Itaconate, which is an unsaturated dicarboxylic acid produced by the decarboxylation of cis-aconitate, is an intermediate metabolite in the tricarboxylic acid cycle and is a striking example of a small metabolite that regulates enzyme activity for cell growth and survival. Initial studies of itaconate production in fungi indicate that the decarboxylation of cis-aconitate to generate itaconate was catalyzed by a ~ 55 kDa protein, which was called cis-aconitate decarboxylase (CAD). In mammals, high amounts of itaconate are produced by macrophages activated by lipopolysaccharide, which is a major pathogen-associated molecular pattern in gram-negative bacteria. Our structural investigation of IRG1 from B. subtilis (bsIRG1) shows that bsIRG1 exhibits the typical fold of the MmgE/PrpD family containing two distinct domains, a helical domain and a lid domain.

The 1.78 Å crystal structure of full-length bsIRG1 was elucidated by using the molecular replacement (MR) method. There were two molecules in the asymmetric unit, chains A and B, both constructed from residues 3 to 445. The structure of bsIRG1 revealed that it consisted of two distinct domains, a helical domain and a lid domain. As the calculated molecular weight of the monomeric full-length bsIRG1 (residues 1 to 445), including the C-terminal His-tag, was 47.7 kDa, the peak generated by the dimer indicated that the working stoichiometry of bsIRG1 is that of a dimer in solution. Unexpectedly, unknown electron density was detected on the side opposite to the active site, between the helical domain and the lid domain, and was assigned to 3-cyclohexyl-1-propylsulfonic acid (CXS) by a ligand identification tool. The main forces involved in CXS binding to bsIRG1 were hydrogen bonds formed between the sulfonic acid moiety of CXS and Y269, R283, and L339 of bsIRG1, and hydrophobic interactions formed between the cyclohexyl group of CXS and the hydrophobic pocket formed by F93, L408, and L419 of bsIRG1. Based on the structural comparison of bsIRG1 with IDS epimerase, mIRG1, and hIRG1, we noticed that bsIRG1 was an open form, whose two loops (A1 and A2) were localized to expose the active site. Structural comparison showed that A1 and A2 loops are flexible and control substrate accessibility by working as a gate. An in silico docking simulation of cis-aconitate and bsIRG1 indicated that C1 and C6 carboxylate groups of cis-aconitate form an extensive network of hydrogen bonds with D91, H102, K200, K266, and C271 from bsIRG1, while C5 carboxylate forms hydrogen bonds only with H151 from bsIRG1. In hIRG1, Y318 performed the role of Y146 of bsIRG1 by interacting with the C6 carboxylate of the substrate.

>[2x]KQGLTAGLAEAVRTSQPEHSVDAIRKAKKGLLDFTAASFAGREDKGIQKLLRLIEDEGGRPLVPIIGQGKKAAPLQSAMLNGFIAHALDFDDVHSDVRGHPSAVIVPALIASAARGHDERLLGAYIVGVEVMARLGESIGSRHYEKGWHNTGTLGAIAAACAVGYAEELTQEELEKAIGFAATQSAGMRVQFGTEMKPLHAGLAAQAGLLAVKLAQSEFGGSRTAFDGETGFFSLYGDVEKAQHTLLNDWGAPWRIVQPGLWFKIYPFCSAAHHAADAVRQLISEETISAANTERIEVIFPPGGDAALTERSPKTGEEGRFSVEYVIALALHGHGLTVEHFSSQPIPNGIQTTIGHIQRVYDNATQPAPHAVPKGRFTIVRAYLSDGRICEARVDCPKGAPGNELSEEDIIEKLTLTVPQEKARRIITAVEKADIKEFLAHIELE> GEKKESETEKSSDIAQVKIKDVSYTLPSKYDKSTSDDQLVLKVNVAVKNTGKDPLNVDSMDFTLYQGDTKMSDTDPEDYSEKLQGSTINADKSVEGNLFFVVDKGKQYELNYTPESYGDKKPKSVTFKIDGKDKKILATADKLQDSAKALSAYVDVLLFGKDNADFEKITGANKNEIV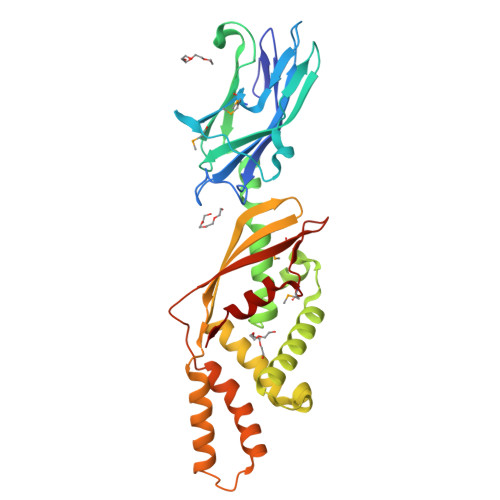NDFNESAKDGYLSASGLSSTYADSKALDNIVNGIKEGLSKNSSIQAKTTSISKDEAIVEATVKPVDASSLSDRIEDKVKDYYSKNSSASYEEAVKYALQVYPEEFKKLGPASSEKTVEVKMKKNDIDQWQLDMDDYRAAELVEAFIKE> MN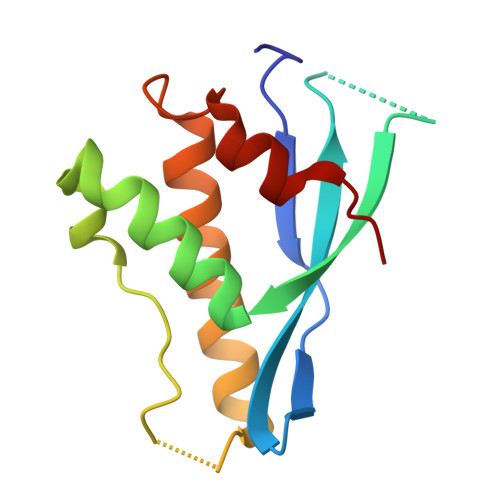LGTWRAVVSTAEASEENGEQMACYFVAVSLSEEDDCKNNHWTVSRKLIEFQALHRKLTECFPSLKKVQLPSLSKLPFKSIDQKFLDKSKNQLNAFLQKVLTDERMCQSEALYAFLSPSLE>[2x]MLRTVTSKTVSNQFKRSLATAVATPKAEVTQLSNGIVVATEHNPSAHTASVGVVFGSGAANENPYNNGVSNLWKNIFLSKENSAVAAKEGLALSSNISRDFQSYIVSSLPGSTDKSLDFLNQSFIQQKANLLSSSNFEATKKSVLKQVQDFEENDHPNRVLEHLHSTAFQNTPLSLPTRGTLESLENLVVADLESFANNHFLNSNAVVVGTGNIKHEDLVNSIESKNLSLQTGTKPVLKKKAAFLGSEVRLRDDTLPKAWISLAVEGEPVNSPNYFVAKLAAQIFGSYNAFEPASRLQGIKLLDNIQEYQLCDNFNHFSLSYKDSGLWGFSTATRNVTMIDDLIHFTLKQWNRLTISVTDTEVERAKSLLKLQLGQLYESGNPVNDANLLGAEVLIKGSKLSLGEAFKKIDAITVKDVKAWAGKRLWDQDIAIAGTGQIEGLLDYMRIRSDMSMMRW;>MLSAARLQFAQGSVRRLTVSARDAPTKISTLAVKVHGGSRYATKDGVAHLLNRFNFQNTNTRSALKLVRESELLGGTFKSTLDREYITLKATFLKDDLPYYVNALADVLYKTAFKPHELTESVLPAARYDYAVAEQCPVKSAEDQLYAITFRKGLGNPLLYDGVERVSLQDIKDFADKVYTKENLEVSGENVVEADLKRFVDESLLSTLPAGKSLVSKSEPKFFLGEENRVRFIGDSVAAIGIPVNKASLAQYEVLANYLTSALSELSGLISSAKLDKFTDGGLFTLFVRDQDSAVVSSNIKKIVADLKKGKDLSPAINYTKLKNAVQNESVSSPIELNFDAVKDFKLGKFNYVAVGDVSNLPYLDEL[2x];>MAFRKSNVYLSLVNSYIIDSPQPSSINYWWNMGSLLGLCLVIQIVTGIFMAMHYSSNIELAFSSVEHIMRDVHNGYILRYLHANGASFFFMVMFMHMAKGLYYGSYRSPRVTLWNVGVIIFILTIATAFLGYCCVYGQMSHWGATVITNLFSAIPFVGNDIVSWLWGGFSVSNPTIQRFFALHYLVPFIIAAMVIMHLMALHIHGSSNPLGITGNLDRIPMHSYFIFKDLVTVFLFMLILALFVFYSPNTLGHPDNYIPGNPLVTPASIVPEWYLLPFYAILRSIPDKLLGVITMFAAILVLLVLPFTDRSVVRGNTFKVLSKFFFFIFVFNFVLLGQIGACHVEVPYVLMGQIATFIYFAYFLIIVPVISTIENVLFYIGRVNK[2x];>MFSNLSKRWAQRTLSKSFYSTATGAASKSGKLTQKLVTAGVAAAGITASTLLYADSLTAEAMTAAEHGLHAPAYAWSHNGPFETFDHASIRRGYQVYREVCAACHSLDRVAWRTLVGVSHTNEEVRNMAEEFEYDDEPDEQGNPKKRPGKLSDYIPGPYPNEQAARAANQGALPPDLSLIVKARHGGCDYIFSLLTGYPDEPPAGVALPPGSNYNPYFPGGSIAMARVLFDDMVEYEDGTPATTSQMAKDVTTFLNWCAEPEHDERKRLGLKTVIILSSLYLLSIWVKKFKWAGIKTRKFVFNPPKPRK[2x];>[2x]MLGIRSSVKTCFKPMSLTSKRLISQSLLASKSTYRTPNFDDVLKENNDADKGRSYAYFMVGAMGLLSSAGAKSTVETFISSMTATADVLAMAKVEVNLAAIPLGKNVVVKWQGKPVFIRHRTPHEIQEANSVDMSALKDPQTDADRVKDPQWLIMLGICTHLGCVPIGEAGDFGGWFCPCHGSHYDISGRIRKGPAPLNLEIPAYEFDGDKVIVG;>[2x]MGMLELVGEYWEQLKITVVPVVAAAEDDDNEQHEEKAAEGEEKEEENGDEDEDEDEDEDDDDDDDEDEEEEEEVTDQLEDLREHFKNTEEGKALVHHYEECAERVKIQQQQPGYADLEHKEDCVEEFFHLQHYLDTATAPRLFDKLK;>MPQSFTSIARIGDYILKSPVLSKLCVPVANQFINLAGYKKLGLKFDDLIAEENPIMQTALRRLPEDESYARAYRIIRAHQTELTHHLLPRNEWIKAQEDVPYLLPYILEAEAAAKEKDELDNIEVSK[2x];>[2x]MGPPSGKTYMGWWGHMGGPKQKGITSYAVSPYAQKPLQGIFHNAVFNSFRRFKSQFLYVLIPAGIYWYWWKNGNEYNEFLYSKAGREELERVNV;>MSFSSLYKTFFKRNAVFVGTIFAGAFVFQTVFDTAITSWYENHNKGKLWKDVKARIAAGDGDDDDE[2x];>[2x]MAYTSHLSSKTGLHFGRLSLRSLTAYAPNLMLWGGASMLGLFVFTEGWPKFQDTLYKKIPLLGPTLEDHTPPEDKPN;> MVQRWLYSTNAKDIAVLYFMLAIFSGMAGTAMSLIIRLELAAPGSQYLHGNSQLFNVLVVGHAVLMIFFLVMPALIGGFGNYLLPLMIGATDTAFPRINNIAFWVLPMGLVCLVTSTLVESGAGTGWTVYPPLSSIQAHSGPSVDLAIFALHLTSISSLLGAINFIVTTLNMRTNGMTMHKLPLFVWSIFITAFLLLLSLPVLSAGITMLLLDRNFNTSFFEVSGGGDPILYEHLFWFFGHPEVYILIIPGFGIISHVVSTYSKKPVFGEISMVYAMASIGLLGFLVWSHHMYIVGLDADTRAYFTSATMIIAIPTGIKIFSWLATIHGGSIRLATPMLYAIAFLFLFTMGGLTGVALANASLDVAFHDTYYVVGHFHYVLSMGAIFSLFAGYYYWSPQILGLNYNEKLAQIQFWLIFIGANVIFFPMHFLGINGMPRRIPDYPDAFAGWNYVASIGSFIATLSLFLFIYILYDQLVNGLNNKVNNKSVIYNKAPDFVESNTIFNLNTVKSSSIEFLLTSPPAVHSFNTPAVQS;> MLDLLRLQLTTFIMNDVPTPYACYFQDSATPNQEGILELHDNIMFYLLVILGLVSWMLYTIVMTYSKNPIAYKYIKHGQTIEVIWTIFPAVILLIIAFPSFILLYLCDEVISPAMTIKAIGYQWYWKYEYSDFINDSGETVEFESYVIPDELLEEGQLRLLDTDTSMVVPVDTHIRFVVTAADVIHDFAIPSLGIKVDATPGRLNQVSALIQREGVFYGACSELCGTGHANMPIKIEAVSLPKFLEWLNEQ;> MTHLERSRHQQHPFHMVMPSPWPIVVSFALLSLALSTALTMH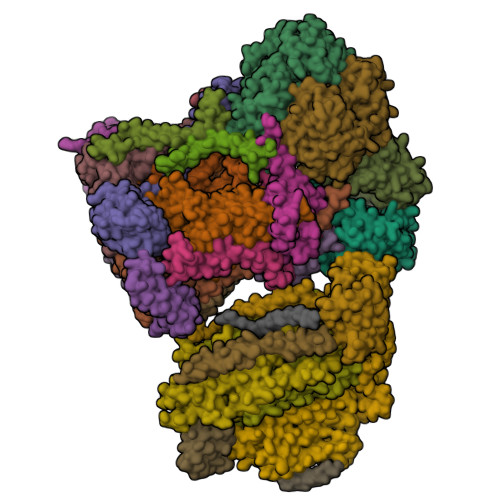GYIGNMNMVYLALFVLLTSSILWFRDIVAEATYLGDHTMAVRKGINLGFLMFVLSEVLIFAGLFWAYFHSAMSPDVTLGACWPPVGIEAVQPTELPLLNTIILLSSGATVTYSHHALIAGNRNKALSGLLITFWLIVIFVTCQYIEYTNAAFTISDGVYGSVFYAGTGLHFLHMVMLAAMLGVNYWRMRNYHLTAGHHVGYETTIIYTHVLDVIWLFLYVVFYWWGV;> MLSLRQSIRFFKPATRTLCSSRYLLQQKPVVKTAQNLAEVNGPETLIGPGAKEGTVPTDLDQETGLARLELLGKLEGIDVFDTKPLDSSRKGTMKDPIIIESYDDYRYVGCTGSPAGSHTIMWLKPTVNEVARCWECGSVYKLNPVGVPNDDHHH;> MLRNTFTRAGGLSRITSVRFAQTHALSNAAVMDLQSRWENMPSTEQQDIVSKLSERQKLPWAQLTEPEKQAVWYISYGEWGPRRPVLNKGDSSFIAKGVAAGLLFSVGLFAVVRMAGGQDAKTMNKEWQLKSDEYLKSKNANPWGGYSQVQSK;> MLSRAIFRNPVINRTLLRARPGAYHATRLTKNTFIQSRKYSDAHDEETFEEFTARYEKEFDEAYDLFEVQRVLNNCFSYDLVPAPAVIEKALRAARRVNDLPTAIRVFEALKYKVENEDQYKAYLDELKDVRQELGVPLKEELFPSSS;> MANKVIQLQKIFQSSTKPLWWRHPRSALYLYPFYAIFAVAVVTPLLYIPNAIRGIKAKKA;> MLCQQMIRTTAKRSSNIMTRPIIMKRSVHFKDGVYENIPFKVKGRKTPYALSHFGFFAIGFAVPFVACYVQLKKSGAF;> MTIAPITGTIKRRVIMDIVLGFSLGGVMASYWWWGFHMDKINKREKFYAELAERKKQEN;> MADQENSPLHTVGFDARFPQQNQTKHCWQSYVDYHKCVNMKGEDFAPCKVFWKTYNALCPLDWIEKWDDQREKGIFAGDINSD;> MFRQCAKRYASSLPPNALKPAFGPPDKVAAQKFKESLMATEKHAKDTSNMWVKISVWVALPAIALTAVNTYFVEKEHAEHREHLKHVPDSEWPRDYEFMNIRSKPFFWGDGDKTLFWNPVVNRHIEHDD2-phenyl-5-(1H-pyrazol-4-yl)-1H-pyrrolo[2,3-b]pyridine 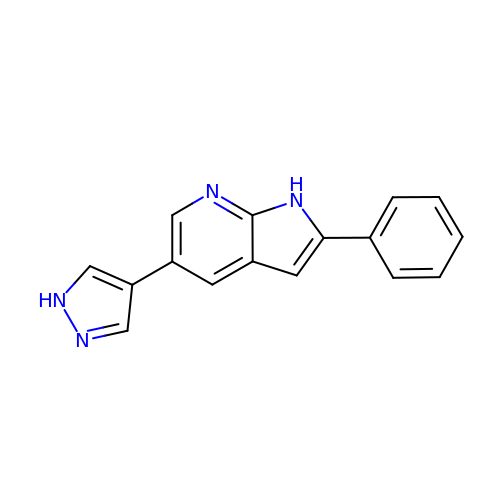| C16 H12 N4 | NSAWQZXLJIAJFT-UHFFFAOYSA-N>[3x]GSPSKEEVMAATQAEGPKRVSDSAIIHTSMGDIHTKLFPVECPKTVENFCVHSRNGYYNGHTFHRIIKGFMIQTGDPTGTGMGGESIWGGEFEDEFH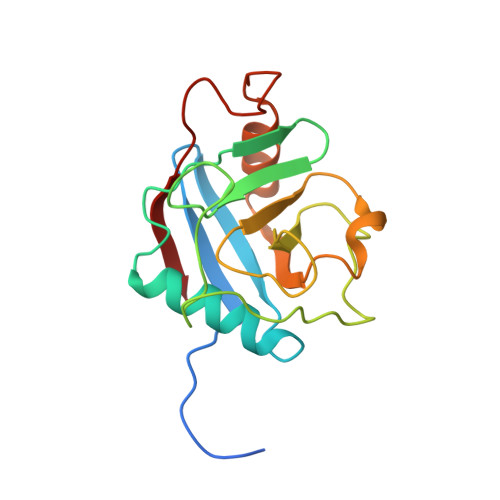STLRHDRPYTLSMANAGSNTNGSQFFITVVPTPWLDNKHTVFGRVTKGMEVVQRISNVKVNPKTDKPYEDVSIINITVK> QIGWRREGIKYRRNELFLDVLESVNLLMSPQGQVLSAHVSGRVVMKSYLSGMPECKFGMNDKIVIEKQGKGTADETSKSGKQSIAIDDCTFHQCVRLSKFDSERSISFIPPDGEFELMRYRTTKDIILPFRVIPLVREVGRTKLEVKVVIKSNFKPSLLAQKIEVRIPTPLNTSGVQVICMKGKAKYKASENAIVWKIKRMAGMKESQISAEIELLPTNDKKKWARPPISMNFEVPFAPSGLKVRYLKVFEPKLNYSDHDVIKWVRYIGRSGIYETRC;> GYMMMSPS

Clathrin-mediated endocytosis (CME) is a major regulator of RTKs involving the heterotetrameric AP2 complex composed of large α and β2, medium μ2, and small σ2 subunits. AP2 binds to transmembrane cargo proteins that contain specific motifs such as YxxΦ (Y denotes Tyr; x, any amino acid; and Φ, bulky hydrophobic residue) serving as μ2 binding sites. In this study, we discovered AP2 is also an IRS-1-associated protein. IRS-1 binds with AP2 to prevent IGF-IR recruitment into clathrin-coated structures and thus enhance surface retention of activated IGF-IR.

We also analyzed the crystal structures of μ2 C-terminal subdomain (C-μ2) bound to IRS-1 YxxΦ motifs. Importantly, the side chains of Tyr and Met residues of IRS-1 YxxΦ motifs are inserted into the binding pockets of μ2, which are shared by the AP2 cargo proteins. Collectively, these results indicate that IRS-1 is recognized by the AP2 complex via the μ2 subunit in the very similar manner to conventional endocytic cargos. Using IRS-1 truncated mutants, we mapped the central region (amino acid residues 543–865) which is necessary for the binding to AP2. This region is almost identical to that for the clathrin adaptor AP1 complex found in our previous study, which binds to YxxΦ motifs of IRS-1 including Tyr 608, Tyr 628, and Tyr 658 via its μ1 subunit. Indeed, the Ala mutation of all these Tyr residues in IRS-1, but not a single substitution, completely abolished the binding to μ2 in vitro (IRS-1 3YA mutant). The Tyr residues of the YxxΦ motifs of IRS-1 (Tyr608, 628, and 658) critical for the binding to AP2 are part of phosphorylation sites among multiple Tyr residues in the C-terminus of IRS-1 that mediate the interaction of IRS-1 with PI3K and subsequent activation of PI3K. In addition, AP2 would preferentially bind non-phosphorylated IRS-1 since AP2 cannot recognize phosphorylated YxxΦ sequence due to its limited capacity. Our results indicate that IRS-1 inhibits the recruitment of IGF-IR to CCPs through YxxΦ motifs in IRS-1.> CGCGAAAACGCG;> CGCGTT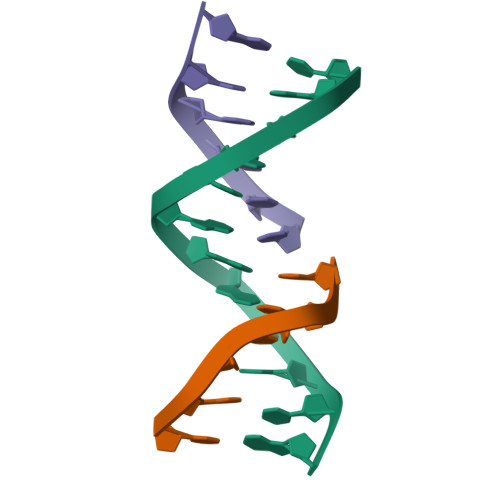;> TTCGCG>[3x]GPLGSDKALKMPASRYLTDMTLEEMSRDWFMLM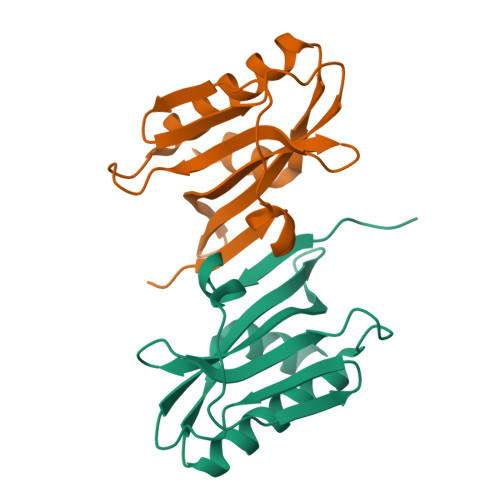PKQKVAGSLCIKMDQAIMDKTIILKANFSVIFDRLETLILLRAFTEEGAIVGEISPLPSLPGHTGEDVKNAIGVLIGGLEANDNTVRVTETIQRFAWRNSDEDGRLPLPPNQKR> MNGVYDVGGTDGLGPINRPADEPVFRAEWEKVAFAMFPATFRAGFMGLDEFAFGIEQMNPAEYLESPYYWHWIRTYIHHGVRTGKIDLEELERRTQYYRENPDAPLPEHEQKPELIEFVNQAVYGGLPASREVDRPPKFKEGDVVRFSTASPKGHARRARYVR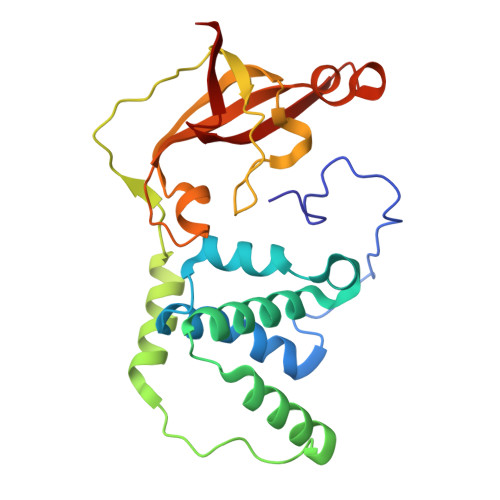GKTGTVVKHHGAYIYPDTAGNGLGECPEHLYTVRFTAQELWGPEGDPNSSVYYDCWEPYIELVDT>[2x]MENTENSVDSKSIKNLEPKIIHGSESMDSGISLDNSYKMDYPEMGLCIIINNKNFHKSTGMTSRSGTDVDAANLRETF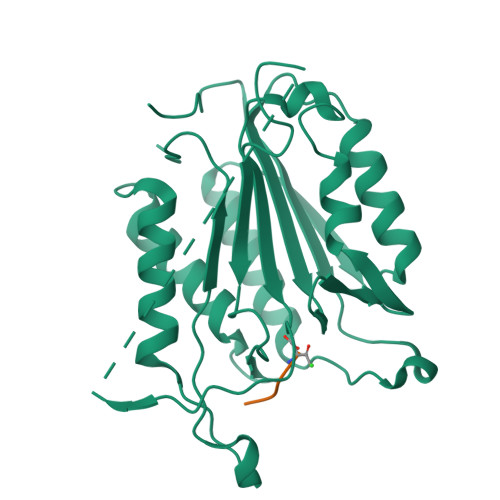RNLKYEVRNKNDLTREEIVELMRDVSKEDHSKRSSFVCVLLSHGEAGIIFGTNGPVDLKKITNFFRGDRCRSLTGKPKLFIIQACRGTELDCGIETDSGVDDDMACHKIPVEADFLYACSTAPGYYSWRNSKDGSWFIQSLCAMLKQYADKLEFMHILTRVNRKVATEFESFSFDATFHAKKQIPCIVSMLTKELYFYH methyl 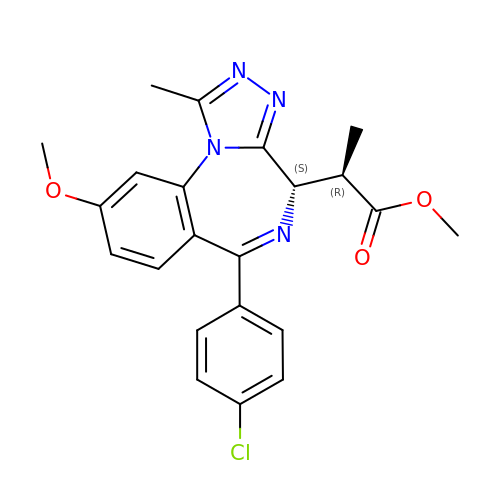(2~{R})-2-[(4~{S})-6-(4-chlorophenyl)-9-methoxy-1-methyl-4~{H}-[1,2,4]triazolo[4,3-a][1,4]benzodiazepin-4-yl]propanoate | C22 H21 Cl N4 O3 | AEUSGDQJZNZQBP-BLVKFPJESA-N> MSANDFKPETWTSSANEALRVSIVGENAVQFSPLFTYPIYGDSEKIYGYKDLIIHLAFDSVTFKPYVNVKYSAKLGDDNIVDVEKKLLSFLPKDDVIVRDEAKWVDCFAEERKTHNLSDVFEKVSEYSLNGEEFVVYKSSLVDDFARRMHRRVQIFSLLFIEAANYIDETDPSWQIYWLLNKKTKELIGFVTTYKYWHYLGAKSFDEDIDKKFRAKISQFLIFPPYQNKGHGSCLYEAIIQSWLEDK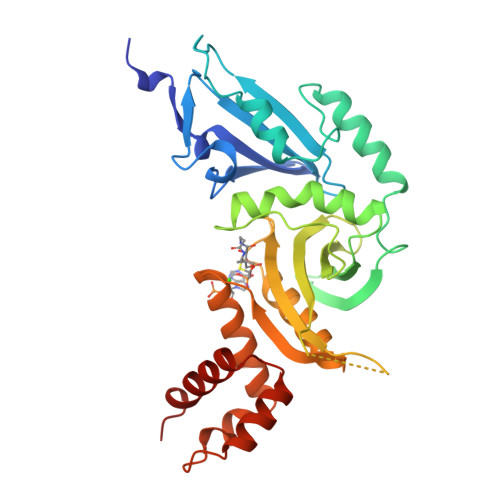SITEITVEDPNEAFDDLRDRNDIQRLRKLGYDAVFQKHSDLSDEFLESSRKSLKLEERQFNRLVEMLLLLNNS>MTYFIDVPTMSDLVHDIGVAPFIGELAAALRDDFKRWQAFDKSARVASHSEVGVIELMPVADKSRYAFKYVNGHPANTARNLHTVMAFGVLADVDSGYPVLLSELTIATALRTAATSLMAAQALARPNARKMALIGNGAQSEFQALAFHKHLGIEEIVAYDTDPLATAKLIANLKEYSGLTIRRASSVAEAVKGVDIITTVTADKAYATIITPDMLEPGMHLNAVGGDCPGKTELHADVLRNARVFVEYEPQTRIEGEIQQLPADFPVVDLWRVLRGETEGRQSDSQVTVFDSVGFALEDYTVLRYVLQQAEKRGMGTKIDLVPWVEDDPKDLFSHTR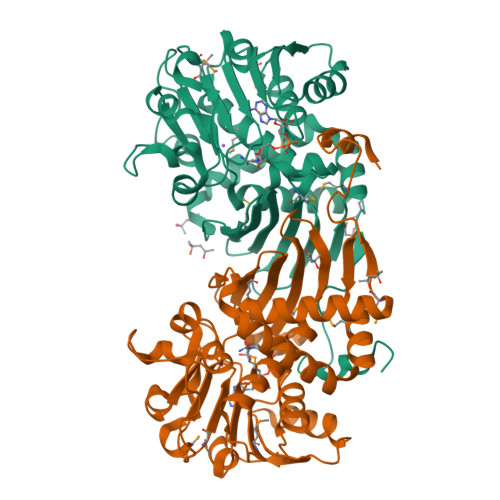GRAGKRRIRRVA[2x]>[4x]MHHHHHHSSGRENLYFQGAAGASMQSAANITLRQILEPNNVNLRSKKTHIVCTLGPACKSVETLVKLIDAGMDICRFNFSHGSHEDHKEMFNNVLKAQELRPNCLLGMLLDTKGPEIRTGFLKNKEVHLKEGSKLKLVTDYEFLGDETCIACSYKKLPQSVKPGNIILIADGSVSCKVLETHEDHVITEVLNSAVIGERKNMNLPNV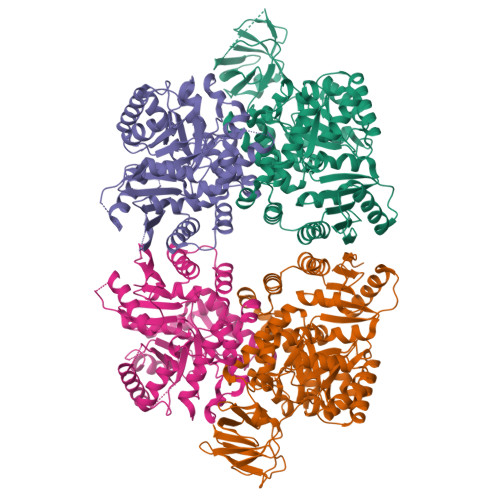KVDLPIISEKDKNDILNFAIPMGCNFIAASFIQSADDVRLIRNLLGPRGRHIKIIPKIENIEGIIHFDKILAESDGIMIARGDLGMEISPEKVFLAQKLMISKCNLQGKPIITATQMLESMTKNPRPTRAEVTDVANAVLDGTDCVMLSGETAGGKFPVEAVTIMSKICLEAEACIDYKLLYQSLVNAIETPISVQEAVARSAVETAESIQASLIIALTETGYTARLIAKYKPSCTILALSASDSTVKCLNVHRGVTCIKVGSFQGTDIVIRNAIEIAKQRNMAKVGDSVIAIHGIKEEVSGGTNLMKVVQIE>[2x]SMQSSKRSSRSVEDDKEGHLVCRIGDWLQERYEIVGNLGEGTFGKVVECLDHARGKSQVALKIIRNVGKYREAARLEINVLKKIKEKDKENKFLCVLMSDWFNFHGHMCIAFELLGKNTFEFLKENNFQPYPLPHVRHMAYQLCHALRFLHENQLTHTDLKPENILF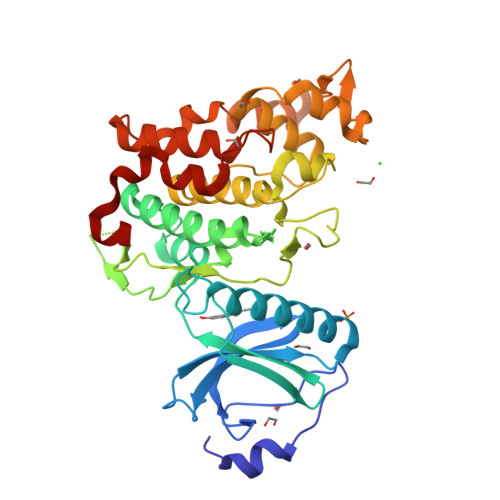VNSEFETLYNEHKSCEEKSVKNTSIRVADFGSATFDHEHHTTIVATRHYRPPEVILELGWAQPCDVWSIGCILFEYYRGFTLFQTHENREHLVMMEKILGPIPSHMIHRTRKQKYFYKGGLVWDENSSDGRYVKENCKPLKSYMLQDSLEHVQLFDLMRRMLEFDPAQRITLAEALLHPFFAGLTPEERSFHT>M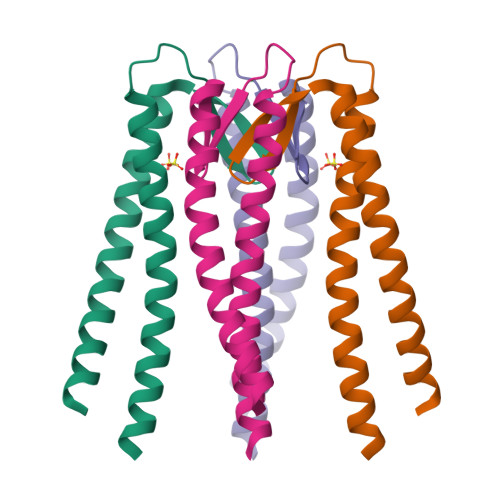EAVRAYELQLELQQIRTLRQSLELKMKELEYAEGIITSLKSERRIYRAFSDLLVEITKDEAIEHIERSRLVYKREIEKLKKREKEIMEELSKLRAPLS[2x]>[2x]FMATIEEIKEVVLKPYTNHRQLTIREVETISINLIDLLI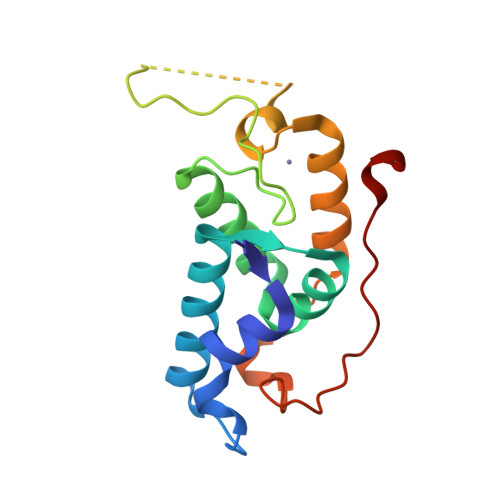TKDVKDARTMKYISRFLTKQDYADLVQERNLVKRCGYPLCSKSQARVRDPFADVQMTNFLRQNNPYAYLTEYCTKAHFRCSQFYQFQLSDEALFARVGVHLDDYEPPSEIQLLEEVLA MONTELUKAST | C35 H36 Cl 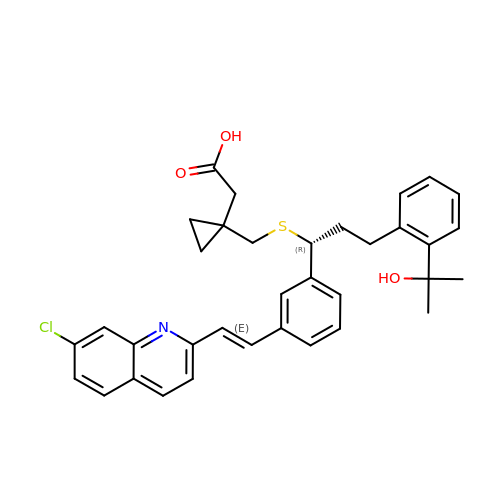N O3 S | UCHDWCPVSPXUMX-TZIWLTJVSA-N>MGNNLMQTDLSVWGMYQHADIVVKCVMIGLILASVVTWAIFFSKSVEFFNQKRRLKREQQLLAEARSLNQANDIAADFGSKSLSLHLLNEAQNELELSEGSDDNEGIKERTSFRLERRVAAVGRQMGRGNGYLATIGAISPFVGLFGTVWGIMNSFIGIAQTQTTNLAVVAPGIAEALLATAIGLVAAIPAVVIYNVFARQIGGFKAMLGDVAAQVLLLQSRDLDLEASAAAHPVRVAQKLRAG[5x];> MTLDLPRRFPWPTLLSVCIHGAVVAGLLYTSVHQVIELPAPAQPISVTMVTPADLEPPQAVQPPPEPVVEPEPEPEPIPEPPKEAPVVIEKPKPKPKPKPKPVKKVQEQPKRDVKPVESRPASPFENTAPARLTSSTATAATSKPVTSVASGPRALSRNQPQYPARAQALRIEGQVKVKFDVTPDGRVDNVQILSAKPANMFEREVKNAMRRWRYEPGKPGSGIVVNILFKINGTTEIQGGGSENLYFQGGSAWSHPQFEK;>[2x]MAMHLNENLDDNGEMHDINVTPFIDVMLVLLIIFMVAAPLATVDVKVNLPASTSTPQP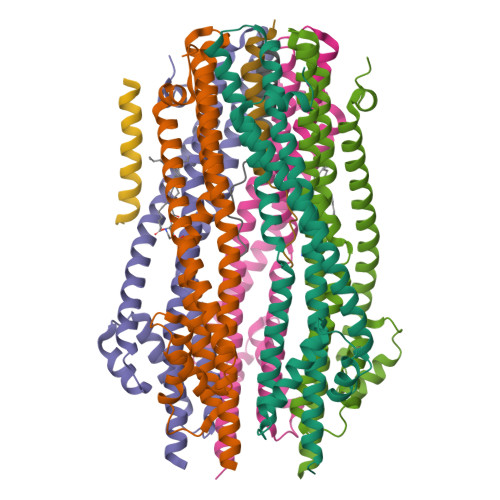RPEKPVYLSVKADNSMFIGNDPVTDETMITALNALTEGKKDTTIFFRADKTVDYETLMKVMDTLHQAGYLKIGLVGEETAKAKENLYFQGNAGSGHHHHHHHHHH Geraniline | C16 H21 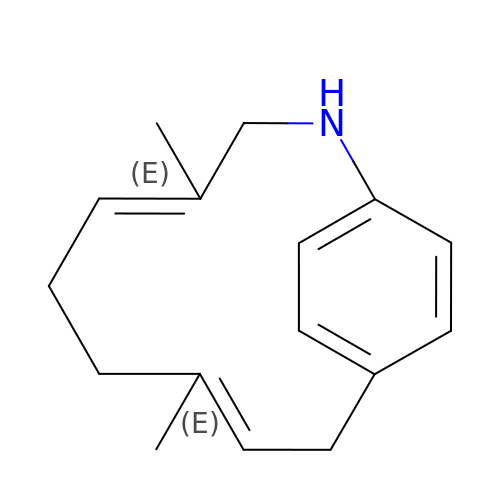N | QEYKICLOTYFCMW-QEKYNVLXSA-N> MLNQELELSLNMAFARAREHRHEFMTVEHLLLALLSNPSAREALEACSVDLVALRQELEAFIEQTTPVLPASEEERDTQPTLSFQRVLQRAV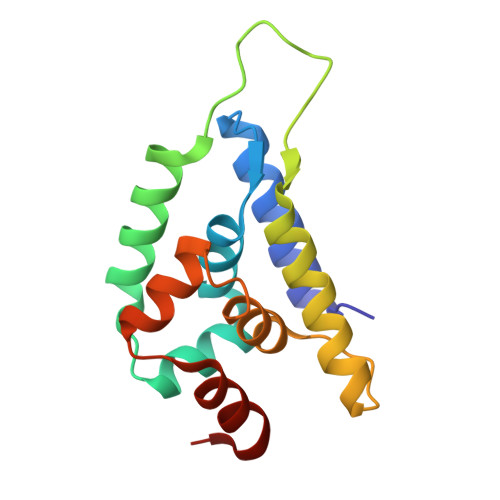FHVQSSGRNEVTGANVLVAIFSEQESQAAYLLRKHEVSRLDVVNFISHGTR> AVTNEEVNQMIEDRKVDFNQNWYFKLNANSKEAIKPDADVSTWKKLDLPYDWSIFNDFDHESPAQNEGGQLNGGEAWYRKTFKLDEKDLKKNVRLTFDGVYMDSQVYVNGQLVGHYPNGYNQFSYDITKYLQKDGRENVIAVHAVNKQPSSRWYSGSG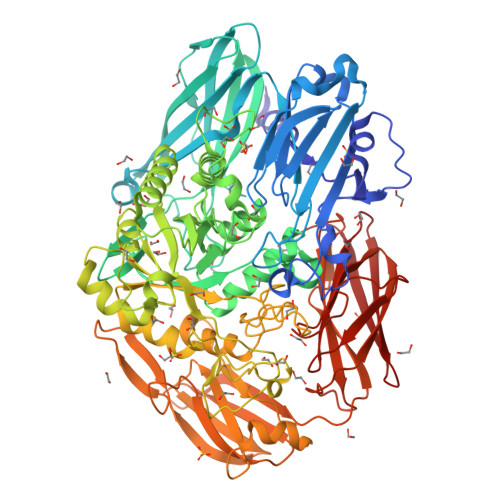IYRDVTLQVTDKVHVEKNGTTILTPKLEEQQHGKVETHVTSKIVNTDDKDHELVAEYQIVERGGHAVTGLVRTASRTLKAHESTSLDAILEVERPKLWTVLNDKPALYELITRVYRDGQLVDAKKDLFGYRYYHWTPNEGFSLNGERIKFHGVSLHHDHGALGAEENYKAEYRRLKQMKEMGVNSIRTTHNPASEQTLQIAAELGLLVQEEAFDTWYGGKKPYDYGRFFEKDATHPEARKGEKWSDFDLRTMVERGKNNPAIFMWSIGNEIGEANGDAHSLATVKRLVKVIKDVDKTRYVTMGADKFRFGNGSGGHEKIADELDAVGFNYSEDNYKALRAKHPKWLIYGSETSSATRTRGSYYRPERELKHSNGPERNYEQSDYGNDRVGWGKTATASWTFDRDNAGYAGQFIWTGTDYIGEPTPWHNQNQTPVKSSYFGIVDTAGIPKHDFYLYQSQWVSVKKKPMVHLLPHWNWENKELASKVADSEGKIPVRAYSNASSVELFLNGKSLGLKTFNKKQTSDGRTYQEGANANELYLEWKVAYQPGTLEAIARDESGKEIARDKITTAGKPAAVRLIKEDHAIAADGKDLTYIYYEIVDSQGNVVPTANNLVRFQLHGQGQLVGVDNGEQASRERYKAQADGSWIRKAFNGKGVAIVKSTEQAGKFTLTAHSDLLKSNQVTVFTGKKEG> MGIVVYTDREVHGAVGSRVTLH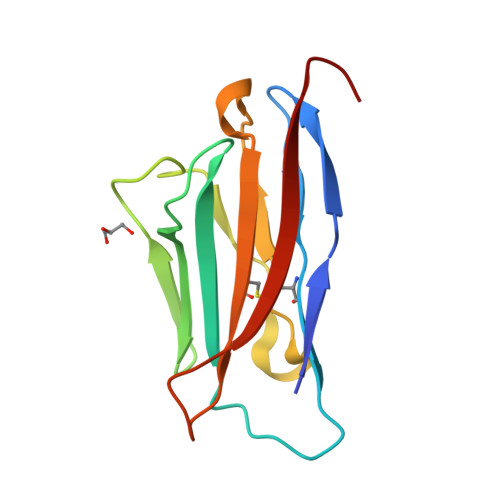CSFWSSEWVSDDISFTWRYQPEGGRDAISIFHYAKGQPYIDEVGTFKERIQWVGDPRWKDGSIVIHNLDYSDNGTFTCDVKNPPDIVGKTSQVTLYVFEKV3-(1,3-thiazol-2-yl)benzoic acid 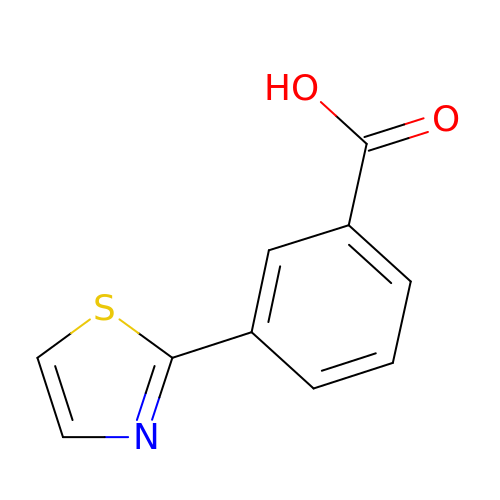| C10 H7 N O2 S | BLFSSABBFANDKK-UHFFFAOYSA-N> MHHHHHHMIEWIIRRSVANRFLVLMGALFLSIWGTWTIINTPVDALPDLSDVQVIIKTSYPGQAPQIVENQVTYPLTTTMLSVPGAKTVRGFSQFGDSYVYVIFEDGTDPYWARSRVLEYLNQVQGKLPAGVSAELGPDATGVGWIYEYALVDRSGKHDLADLRSLQDWFLKYELKTIPDVAEVASVGGVVKEYQVVIDPQRLAQYGISLAEVKSALDASNQEAGGSSIELAEAEYMVRASGYLQTLDDFNHIVLKASENGVPVYLRDVAKVQIGPEMRRGIAELNGEGEVAGGVVILRSGKNAREVIAAVKDKLETLKSSLPEGVEIVTTYDRSQLIDRAIDNLSGKLLEEFIVVAVVCALFLWHVRSALVAIISLPLGLCIAFIVMHFQGLNANIMSLGGIAIAVGAMVDAAIVMIENAHKRLEEWQH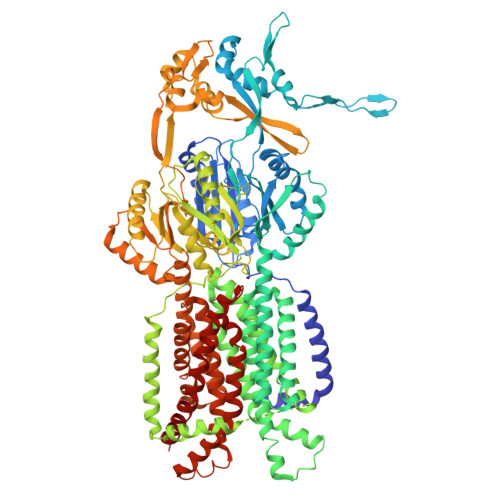QHPDATLDNKTRWQVITDASVEVGPALFISLLIITLSFIPIFTLEGQEGRLFGPLAFTKTYAMAGAALLAIVVIPILMGYWIRGKIPPESSNPLNRFLIRVYHPLLLKVLHWPKTTLLVAALSVLTVLWPLNKVGGEFLPQINEGDLLYMPSTLPGISAAEAASMLQKTDKLIMSVPEVARVFGKTGKAETATDSAPLEMVETTIQLKPQEQWRPGMTMDKIIEELDNTVRLPGLANLWVPPIRNAIDMLSTGIKSPIGIKVSGTVLADIDAMAEQIEEVARTVPGVASALAERLEGGRYINVEINREKAARYGMTVADVQLFVTSAVGGAMVGETVEGIARYPINLRYPQSWRDSPQALRQLPILTPMKQQITLADVADIKVSTGPSMLKTENARPTSWIYIDARDRDMVSVVHDLQKAIAEKVQLKPGTSVAFSGQFELLERANHKLKLMVPMTLMIIFVLLYLAFRRVGEALLIISSVPFALVGGIWLLWWMGFHLSVATGTGFIALAGVAAEFGVVMLMYLRHAIEAVPSLNNPQTFSEQKLDEALYHGAVLRVRPKAMTVAVIIAGLLPILWGTGAGSEVMSRIAAPMIGGMITAPLLSLFIIPAAYKLMWLHRHRVRK> MPVRQPTQGGVQVPGLTGYQSAGVAQPVYRAPQEEAQGVSQFWQNLLPASVKTAQAAQQTASAKGYLEGQQDSQQGREKQVRNFFTKEAYEQGYNSASVNSALASFQLGLQNTAQQYVNSGKTPEEFNVHVQQQTNQLLQEAGAQGLNLNDKDWQAWLGSVEHSRNTANASYQDLNLKRAAVLQEQSWGARGNAAIADFVTAQQSGDTEQALQNVNSFISSVTHDDSITAENKIKYTSQFVVNAFANANSTGDMQALTGYVQSLSEFKNMPTDVQTQIMGSAQQYYQQRASDESVQLYEYNSRVNSVTDYKTLNEAYPMAQYIGTVMQAVQQKKLSPGTGYGMVDAESQRRLKMQKAEQGQLAYTNGVTISDIAAGTGESLDKVKGELTKMYATIGQGYSGGGLQLMQRGLKSGAQDITGVGIEMMQQDAQSLSGIDWRNLKTDADGKPLYPAAVVGSLGNLQAAYQSALAAGNQVQANQLLSGLPDPVVYGIRQNVDARDLADVVGKRAQDIASGKVLALPANMPADVSITQADVTAGIFDLGLGKDARNRNMLGIQSWVFTSDADEKAAQARVSQVNSAMNNEYVYNQQRGSLPALVGDDLKSWLMGKVASRTVRVKDGTDNGALLVLPEVGDKQKVFGSTDNGIIESALTESVTNFKKQYPQATTVQMDYDPLTQELIFQGVNAENQLGTTRASIPAADFRNTVRGVQNTLTQNGSGTTQGNLNVPGAGFVSFNAGNSFGIQKNVVM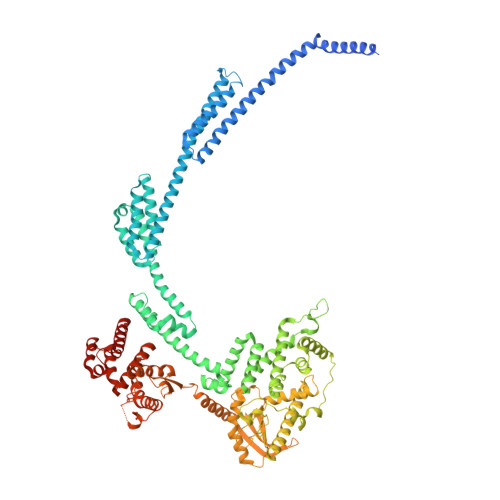GAVNQLVSYEGYTPSKGFSVLGVHPTTGAKLNEDKYVKQATDTPQVAADKFNMYLNDKVYPLVMPKMEQYKNLPGYIQNNIYNALVETTYHSGNSDVFDKYIQTALYGNVQEIPTFKDTPLFKDAGAGSRRNVDRYQLLGSLVTYRTNNPNLSK> HHDITFRNIRFRYKPDSPVILDNINLSIKQGEVI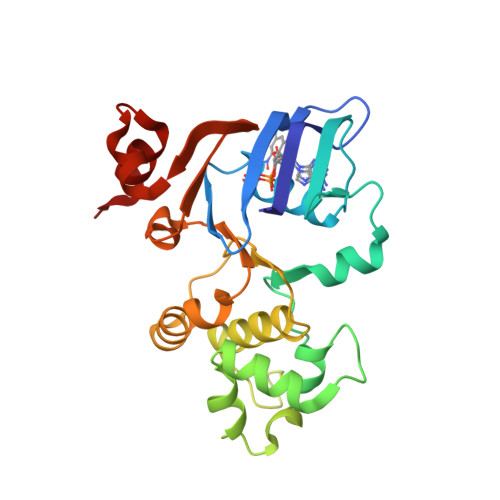GIVGRSGSGKSTLTKLIQRFYIPENGQVLIDGHDLALADPNWLRRQVGVVLQDNVLLNRSIIDNISLANPGMSVEKVIYAAKLAGAHDFISELREGYNTIVGEQGAGLSGGQRQRIAIARALVNNPKILIFDEATSALDYESEHVIMRNMHKICKGRTVIIIAHRLSTVKNADRIIVMEKGKIVEQGKHKELLSEPESLYSYLYQLQSD3-[(2,4-DICHLOROPHENYL)METHYLSULFANYLMETHYL]BENZOIC ACID 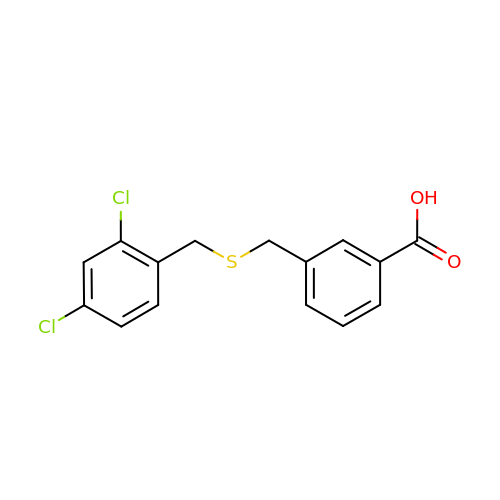| C15 H12 Cl2 O2 S | HGKCARZTNCHYIF-UHFFFAOYSA-N> MGSDKIHHHHHHENLYFQGMSSKQHCVKLNDGHLIPALGFGTYKPKEVPKSKSLEAACLALDVGYRHVDTAYAYQVEEEIGQAIQSAIAAGVVKREDLFVTTKLWCT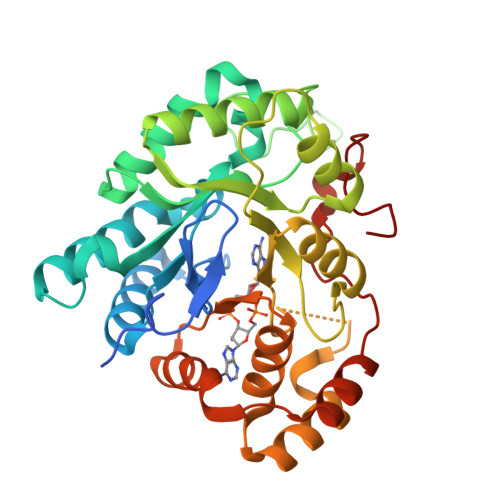CFRPELVKPALEKSLKKLQLDYVDLYIMHYPVPMKSGDNDFPVNEQGKSLLDTVDFCDTWERLEECKDAGLVKSIGVSNFNHRQLERILNKPGLKYKPVCNQVECHLYLNQRKLLDYCESKDIVLVAYGALGTQRYKEWVDQNSPVLLNDPVLCDVAKKNKRSPALIALRYLIQRGIVPLAQSFKENEMRENLQVFGFQLSPEDMKTLDGLNKNFRYLPAEFLVDHPEYPFVEEY>MQKIGIYPGTFDPVTNGHIDIIHRSSELFEKLIVAVAHSSAKNPMFSLDERLKMIQLATKSFKNVECVAFEGLLANLAKEYHCKVLVRGLRVVSDF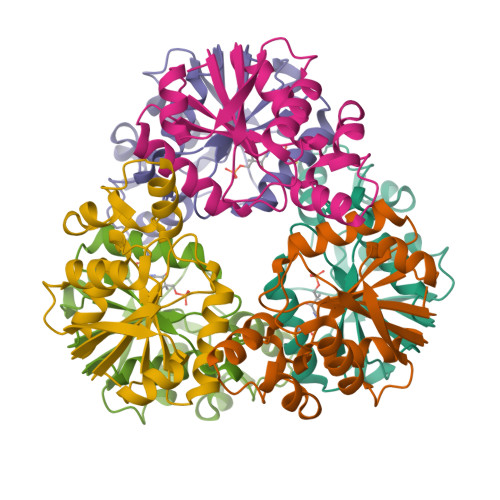EYELQMGYANKSLNHELETLYFMPTLQNAFISSSIVRSIIAHKGDASHLVPKEIYPLISKA[2x]> RPQGATVSLWETVQKWREYRRQCQRSLTEDPPPATDLFCNRTFDEYACWPDGEPGSFVNVSCPWYLPWASSVPQGHVYRF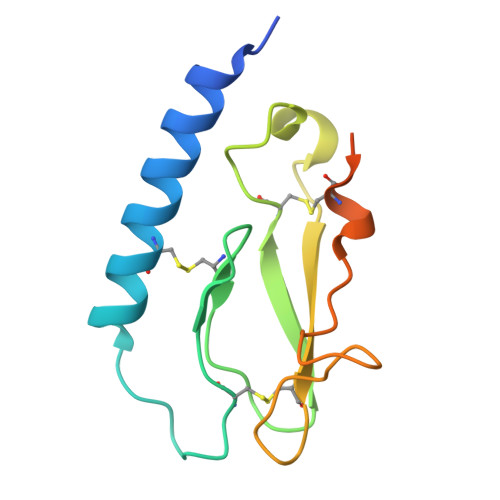CTAEGLWLQKDNSSLPWRDLSECEESKRGERSSPEEQLLFLY> GDVLSTHLDDARRQHIAEKTGKILTEFLQFYEDQYGVALFNSMRHEIEGTGLPQAQLLWRKVPLDERIVFSGNLFQHQEDSKKWRNRFSLVPHNYGLVLYENKAAYERQVPPRAVINSAGYKILTSVDQYLELIGNSLPGTTAKSGSAPILKCPTQFPLILWHPYARHYYFCMMTEAEQDKWQAVLQDCIRHCNNGIPEDSKVEGPAFTDAIRMYRQSKELYGTWEMLCGNEVQILSNLVMEELGPELKAELGPRLKGKPQERQRQWIQISDAVYHMVYEQAKARFEEVLSKVQQVQPAMQAV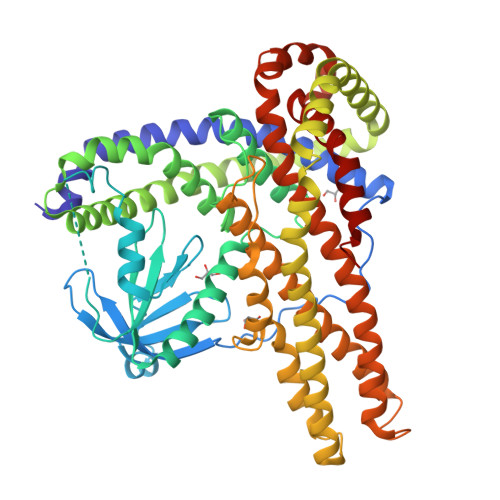IRTDMDQIITSKEHLASKIRAFILPKAEVCVRNHVQPYIPSILEALMVPTSQGFTEVRDVFFKEVTDMNLNVINEGGIDKLGEYMEKLSRLAYHPLKMQSCYEKMESLRLDGLQQRFDVSSTSVFKQRAQIHMREQMDNAVYTFETLLHQELGKGPTKEELCKSIQRVLERVLKKYDYDSSSVRKRFFREALLQISIPFLLKKLAPTCKSELPRFQELIFEDFARFILVENTYEEVVLQTVMKDILQAVKEAAVQR Methylation catalysed by catechol-O-methyltransferase (COMT) is the main pathway of catechol neurotransmitter deactivation in the prefrontal cortex. COMT is a single-domain Mg2+-dependent methyltransferase that catalyses the transfer of an activated methyl group from S-adenosylmethionine (SAM) to its catechol substrate. The crystal structure of COMT comprises a central β-sheet flanked by α-helices, constructing a bipartite active site that accommodates the methyl donor SAM (in the so-called adenine site) and that can also complex an Mg2+ ion to which the catechol substrates bind. Here, a set of apo, semi-holo, holo and Michaelis form crystal structures are described that define the conformational space available to COMT and that include likely intermediates along the catalytic pathway.

We have determined such structures for rat COMT in a variety of conditions and crystal forms. Water replaces Mg2+ and is contacted by Asp184 and Asp212. The β5/α9 loop has now swung out to its maximum extent. In the open state neither the adenine site nor the Mg2+ site are formed. Residues His185, Trp186 and Arg189 stack on top of each other, with Trp186 occupying the usual position of the adenine base. In the absence of a ribose, Glu133 hydrogen-bonds to the indole N atom of Trp186. The different sequences, crystallization conditions and crystal settings all indicate that this form is a recurring state of apo COMT.

>[4x]MGDTKEQRILRYVQQNAKPGDPQSVLEAIDTYCTQKEWAMNVGDAKGQIMDAVIREYSPSLVLELGAYCGYSAVRMARLLQPGARLLTMEMNPDYAAITQQMLNFAGLQDKVTILNGASQDLIPQLKKKYDVDTLDMVFLDHWKDRYLPDTLLLEKCGLLRKGTVLLADNVIVPGTPDFLAYVRGSSSFECTHYSSYLEYMKVVDGLEKAIYQGPSSPDKS Here, we explore the precise structural inhibitory mechanism of actinonin, which is a slow, tight-binding inhibitor of peptide deformylase (PDF), a metal cation-dependent enzyme. PDF is the first enzyme in the N-terminal methionine excision pathway, an essential and ubiquitous process that contributes to the diversity of N-terminal amino acids. The function of the active-site metal is to activate the reactive water molecule involved in peptide hydrolysis. Actinonin is a natural product with antibiotic activity that inhibits PDF by mimicking the structure of its natural substrates (nascent peptide chains starting with Fo-Met-Aaa, where Fo is a formyl group and Aaa is any amino acid) in their transition state.

Compound 21 corresponds to another interesting derivative designed to probe the impact of the peptide bond in PDF binding. In addition to the hydroxamate group, this compound features both a hydrophobic benzyl group at P1' and a reverse peptide bond. Compound 21 shows modest but significant inhibitory potency to AtPDF1B (KI*  = 400±37 nM), confirming the crucial role of the peptide bond in PDF binding. After soaking with crystals of apo-AtPDF, compound 21 could be detected in high-resolution electron density maps. Unlike 6b, 21 did not bind the active site of the enzyme but an alternative pocket at the surface of the protein. A docking study performed with EcPDF had previously revealed this alternative binding pocket. Upon binding of 21, the 3D structure of both molecules of the asymmetric unit remain in an O conformation (r.m.s.d. <0.2 Å with respect to the apo-structures in the “O” state). This finding suggests that only the binding of compounds entering the S1' pocket, such as actinonin or 6b, induces conformational change, in keeping with the crucial role of the P1' group if located in the frame of a classic peptide bond. Moreover, we noticed that the binding pocket of 21 was located on the rear side of the true S1' pocket and induced a weak modification of the P1' hosting platform.

>[2x]MEIVEYPDPILRAKNKRIDIFDENLKNLVDAMFDVMYKTDGIGLSAPQVGLNVQLMVFNPAGEPGEGKEIVLVNPKIKKYSDKLVPFDEGCLSFPGIYAEVVRPQSVKIDARDITGERFSISLSRLPARIFQHEYDHLEGVLFFDRMTDQVLDSIREELEALEKKYEEKTGLPSPERVEARQKRKAGVGFGKR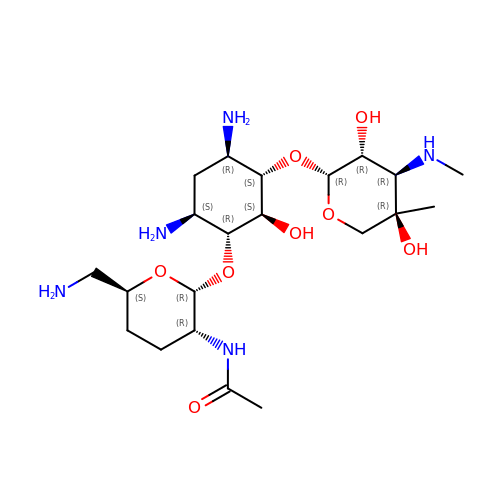(1R,2S,3S,4R,6S)-4,6-diamino-3-{[3-deoxy-4-C-methyl-3-(methylamino)-beta-L-arabinopyranosyl]oxy}-2-hydroxycyclohexyl 2-(acetylamino)-6-amino-2,3,4,6-tetradeoxy-alpha-D-erythro-hexopyranoside | C21 H41 N5 O8 | RLGSXXMFPPOROB-JOYMZIHVSA-N> QLMEGNGPAAVHYQPASPPRDACVYSSCYSEENVWKLCEYIKNHDQYPLEECYAVFISNERKMIPIWKQQARPGDGPVIWDYHVVLLHVSSGGQSFIYDLDTVLPFPCLFDTYVEDAIKSDDDIHPQFRRKFRVICADSYLKNFASDRSHMKDSSGNWRE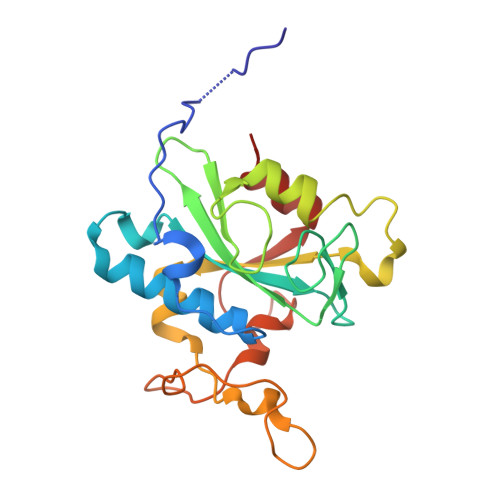PPPPYPCIETGDSKMNLNDFISMDPKVGWGAVYTLSEFTHRFGS>[3x]MEESSEIKVETNISKTSWIRSSMAASGKRVSKALSYITGEMKECGEGLKDKSPVFQFFDWVLRGTSQVMFVNNPLSGILIILGLFIQNPWWAISGCLGTIMSTLTALILSQDKSAIAAGFHGYNGVLVGLLMAVFSDKGDYYWWLLLPVIIMSMSCPILSSALGTIFSKWDLPVFTLPFN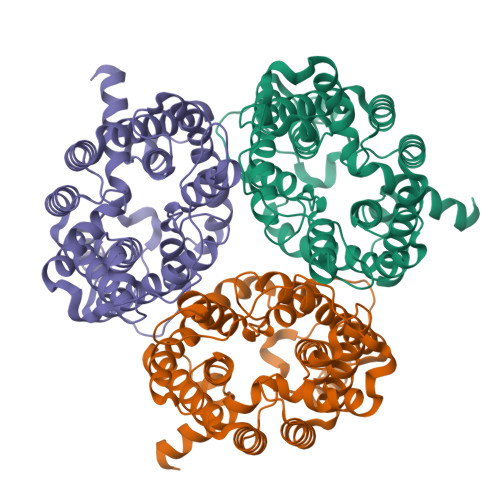ITVTLYLAATGHYNLFFPTTLLQPASAMPNITWSEVQVPLLLRAIPVGIGQVYGCDNPWTGGIFLIALFISSPLICLHAAIGSTMGMLAALTIATPFDSIYFGLCGFNSTLACIAIGGMFYVITWQTHLLAIACALFAAYLGAALANMLSVFGLPPCTWPFCLSALTFLLLTTNNPAIYKLPLSKVTYPEANRIYYLSQERNRRASIITKYQAYDVS>GSIEIPMDLTQPPTITKQSVKDHIVDPRDNILIECEAKGNPAPSFHWTRNSRFFN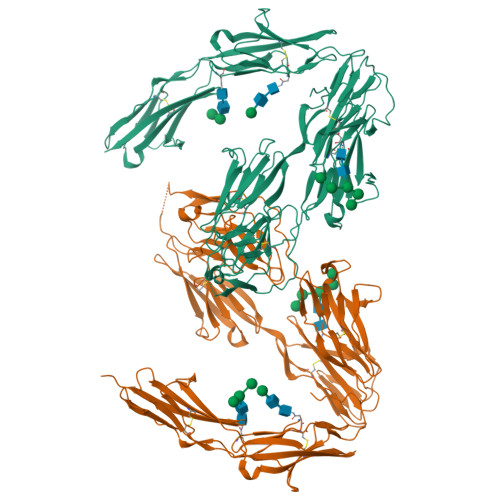IAKDPRVSMRRRSGTLVIDFRSGGRPEEYEGEYQCFARNKFGTALSNRIRLQVSKSPLWPKENLDPVVVQEGAPLTLQCNPPPGLPSPVIFWMSSSMEPITQDKRVSQGHNGDLYFSNVMLQDMQTDYSCNARFHFTHTIQQKNPFTLKVLTNNPYNDSSLRNHPDIYSARGVAERTPSFMYPQGTSSSQMVLRGMDLLLECIASGVPTPDIAWYKKGGDLPSNKAKFENFNKALRITNVSEEDSGEYFCLASNKMGSIRHTISVRVKAAPYWLDEPKNLILAPGEDGRLVCRANGNPKPTVQWMVNGEPLQSAPPNPNREVAGDTIIFRDTQISSRAVYQCNTSNEHGYLLANAFVSVLDVPPRMLSARNQLIRVILYNRTRLDCPFFGSPIPTLRWFKNGQGSNLDGGNYHVYENGSLEIKMIRKEDQGIYTCVATNILGKAENQVRLEVKDPTRIYRMPEDQVAKRGTTVQLECRVKHDPSLKLTVSWLKDDEPLYIGNRMKKEDDSLTIFGVAERDQGSYTCMASTELDQDLAKAYLTVLADQATPTNRLAAHHHHHH[2x]> LSAASWRTQSIYFLLTDRFGRTDNSTTATCNTGNEIYCGGSWQGIIDHLDYI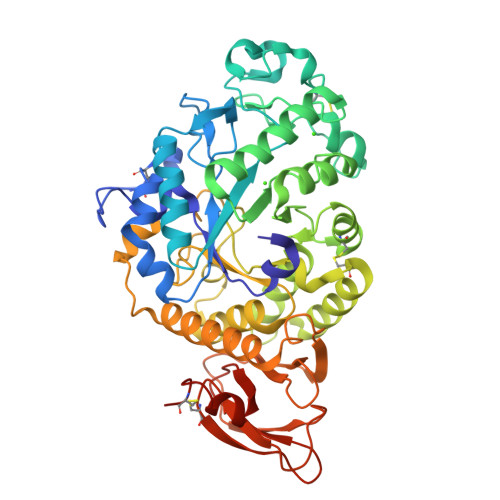EGMGFTAIWISPITEQLPQDTADGEAYHGYWQQKIYDVNSNFGTADNLKSLSDALHARGMYLMVDVVPDHMGYAGNGNDVDYSVFDPFDSSSYFHPYCLITDWDNLTMVEDCWEGDTIVSLPDLDTTETAVRTIWYDWVADLVSNYSVDGLRIDSVLEVQPDFFPGYNKASGVYCVGEIDNGNPASDCPYQKVLDGVLNYPIYWQLLYAFESSSGSISNLYNMIKSVASDCSDPTLLGNFIENHDNPRFAKYTSDYSQAKNVLSYIFLSDGIPIVYAGEEQHYAGGKVPYNREATWLSGYDTSAELYTWIATTNAIRKLAIAADSAYITYANDAFYTDSNTIAMAKGTSGSQVITVLSNKGSSGSSYTLTLSGSGYTSGTKLIEAYTCTSVTVDSSGDIPVPMASGLPRVLLPASVVDSSSLCGGSGRLYVE>[2x]MQGVNIYNISAGTSVDLAAPVTTGDIVTFFSSALNLNA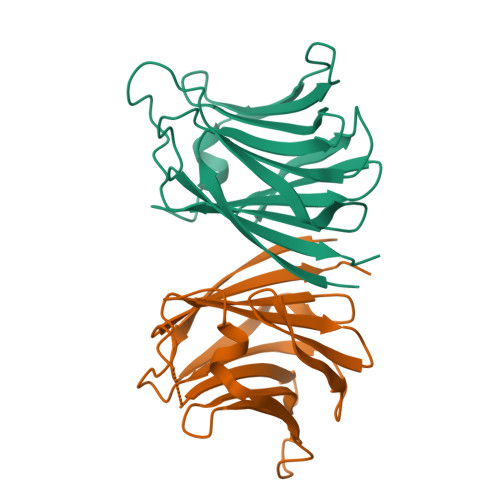GAGNPNNTTLNLFAENGAYLLHIAFRLQENVIIFNSRQPDGPWLVEQRVSDVANQFAGIDGKAMVTVFDHGDKYQVVINEKTVIQYTKQISGLTSSLSYNATEETSGFSTVVEAVTYTGLALEHHHHHH>MGEKCGPPPPIDNGDITSFLLSVYAPGSSVEYQCQNLYQLEGNNQITCRNGQWSEPPKC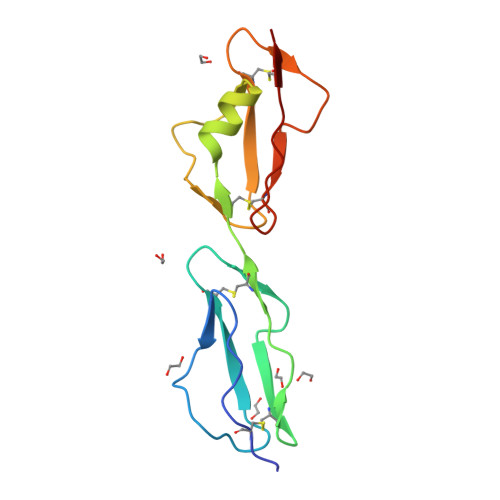LDPCVISQEIMEKYNIKLKWTNQQKLYSRTGDIVEFVCKSGYHPTKSHSFRAMCQNGKLVYPSCEEK[2x]5'-deoxy-5'-({(2S)-2-({2-[(N-{(2R)-4-[(dioxo-lambda~5~-phosphanyl)oxy]-2-hydroxy-3,3-dimethylbutanoyl}-beta-alanyl)amino]ethyl}sulfanyl)-2-[(2S)-pyrrolidin-2-yl]ethanesulfonyl}amino)adenosine 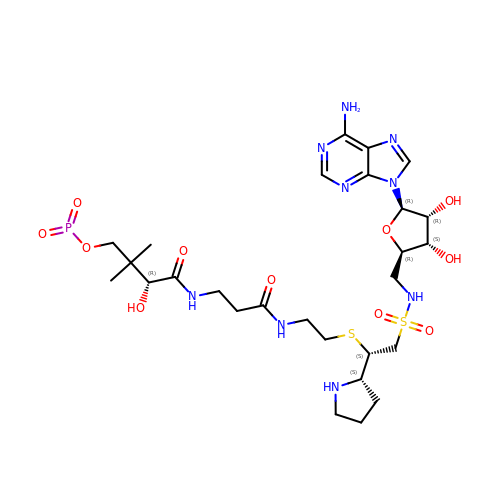| C27 H44 N9 O11 P S2 | UUZQPBPCNSKBOR-LCZLERPASA-N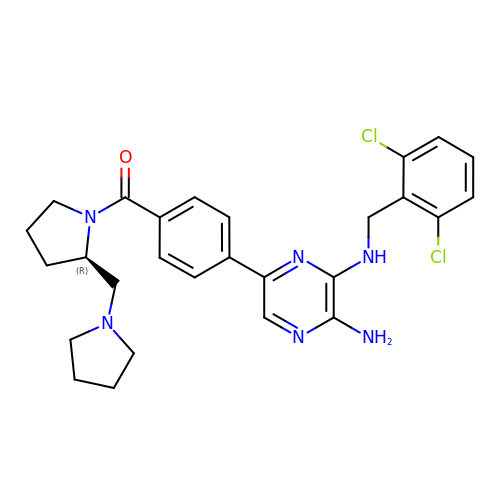N~3~-(2,6-dichlorobenzyl)-5-(4-{[(2R)-2-(pyrrolidin-1-ylmethyl)pyrrolidin-1-yl]carbonyl}phenyl)pyrazine-2,3-diamine | C27 H30 Cl2 N6 O | PVBCEWZVPUKFNT-HXUWFJFHSA-N>[3x]MCGIVGAIAQRDVAEILLEGLRRLEYRGYDSAGLAVVDAEGHMTRLRRLGKVQMLAQAAEEHPLHGGTGIAHTRWATHGEPSEVNAHPHVSEHIVVVHNGIIENHEPLREELKARGYTFVSETDTEVIAHLVNWELKQGGTLREAVLRAIPQLRGAYGTVIMDSRHPDTLLAARSGSPLVIGLGMGENFIASDQLALLPVTRRFIFLEEGDIAEITRRSVNIFDKTGAEVKRQDIESNLQYDAGDKGIYRHYMQKEIYEQPNAIKNTLTGRISHGQ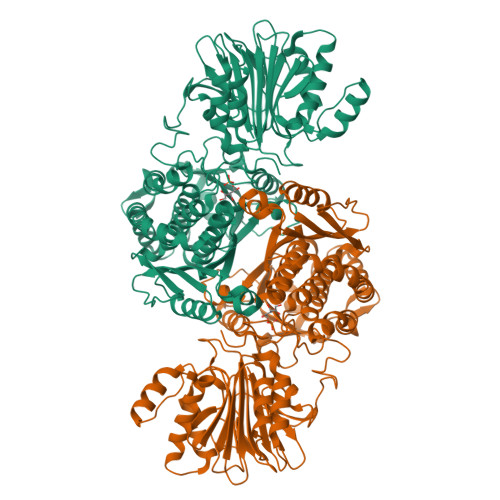VDLSELGPNADELLSKVEHIQILACGTSYNSGMVSRYWFESLAGIPCDVEIASEFRYRKSAVRRNSLMITLSQSGETADTLAGLRLSKELGYLGSLAICNVPGSSLVRESDLALMTNAGTEIGVASTKAFTTQLTVLLMLVAKLSKLKGLDASIEHDIVHGLQALPSRIEQMLSQDKRIEALAEDFSDKHHALFLGRGDQYPIALEGALKLKEISYIHAEAYAAGELKHGPLALIDADMPVIVVAPNNELLEKLKSNIEEVRARGGQLYVFADQDAGFVSSDNMHIIEMPHVEEVIAPIFYTVPLQLLAYHVALIKGTDVDQPRNLAKSVTVE> MDTLEGSMAQLKKGLESGTVLIQFEQLYRKKPGLAITFAKLPQNLDKNRYKDVLPYDTTRVLLQGNEDYINASYVNMEIPAANLVNKYIATQGPLPHTCAQFWQVVWDQKLSLIVMLTTLTERGRTKCHQYWPDPPDVMNHGGFHIQ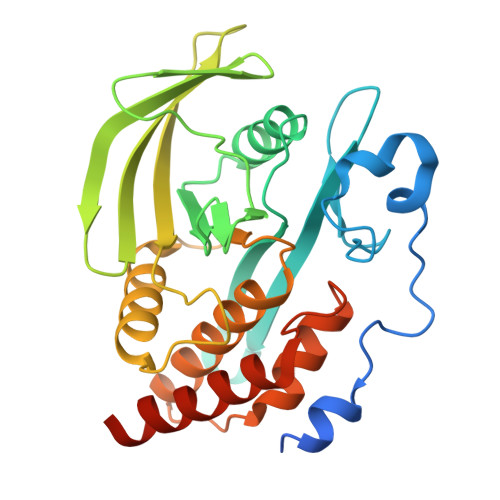CQSEDCTIAYVSREMLVTNTQTGEEHTVTHLQYVAWPDHGVPDDSSDFLEFVNYVRSLRVDSEPVLVHCSAGIGRTGVLVTMETAMCLTERNLPIYPLDIVRKMRDQRAMMVQTSSQYKFVCEAILRVYEEGLVQMLDPS> HPETLVKVKDAEDQLGGRVGYIELDLASGKILESFRPEERFPMMSTFKVLLCGAVLSRVDAGQEQLGRRIHYSQNDLVEYSPVTEKHLTDGMTVGELCSAAITMSDNTAANLLLTTIGGPKELTAFLHNMGDHVTRLDSWEPELNEAIPNDERDTTTPVAMATTLRKLLTGELLTAASRQQLIDWMEADKVA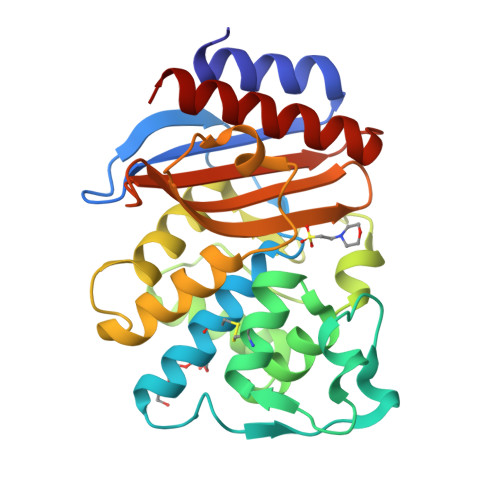GPLLRSALPAGWFIADKSGAGERGSRGIIAALGPDGKPSRIVVIYMTGSQATMDERNRQIAEIGASLIKHW>GAP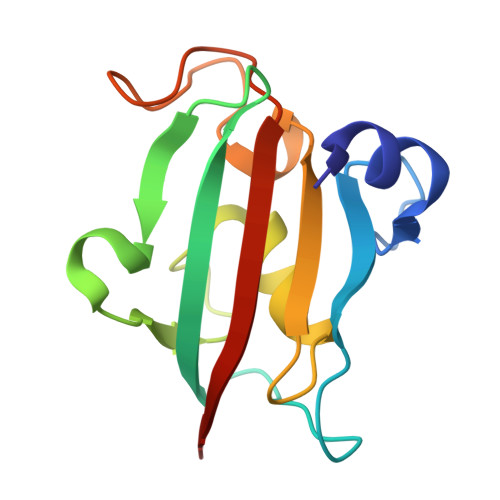ATVAEQGEDITSKKDRGVLKIVKRVGNGEETPMIGDKVYVHYKGKLSNGKKFDSSHDRNEPFVFSLGKGQVIKAWDIGVATMKKGEICHLLCKPEYAYGSAGSLPKIPSNATLFFEIELLDFKGE[4x]>[2x]MDPSVTLWQFLLQ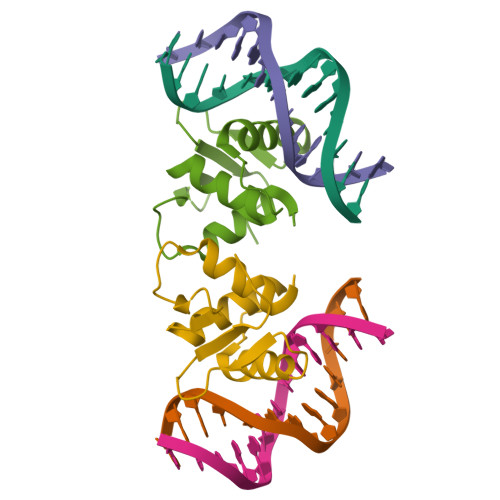LLREQGNGHIISWTSRDGGEFKLVDAEEVARLWGLRKNKTNMNYDKLSRALRYYYDKNIIRKVSGQKFVYKFVSYPEVAGC> ADGKA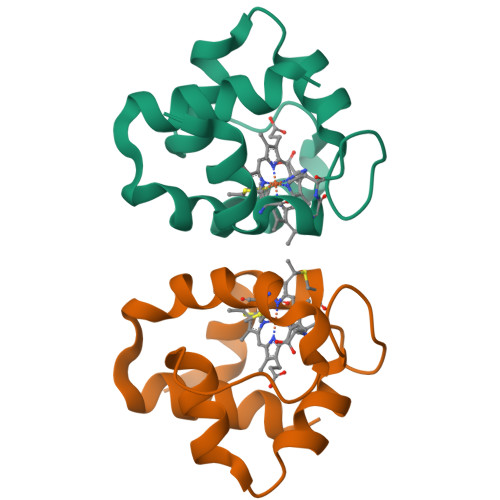IFQQKGCGSCHQANVDTVGPSLKKIAQAYAGKEDQLIKFLKGEAPAIVDPAKEAIMKPQLTMLKGLSDAELKALADFILSHK However, amongst these remodelers, the INO80 chromatin remodeler appears largely sufficient to generate the well positioned +1 and −1 nucleosomes. S.c INO80 is a multi-subunit complex consisting of 15 subunits that are divided into three different modules. The catalytic module with the Ino80 (ATPase) RecA lobes and insert, Arp5, Ies6, Ies2, Rvb1 and Rvb2, constitutes the core unit of INO80 (C-module). INO80 slides nucleosomes with 40 bp of flanking DNA ~100-fold slower than nucleosomes with 80 bp of flanking DNA, displaying a switch like response to flanking DNA length.

To assess whether the nucleotide state affected the location of the Arp8 module, we determined structures of S.c INO80 on 0/80 and 0/40 nucleosomes in the presence of a non-hydrolysable ATP analog (ADP/BeFx). The overall structure of INO80 bound to 0/80 nucleosomes in the presence of ADP/BeFx is similar to the previously published structure in the apo state. The INO80 C-module is well resolved at a resolution of 2.8 Å. The Arp8 module is resolved as a well-defined density on the flanking DNA (~40 bp). Although at a lower resolution (~11.2 Å), we can dock the previously published atomic model of the S.c Arp8 module bound to the HSA region of the ATPase into this density. For X.l nucleosomes, no difference is observed between the previously published structure in the apo state and the structure determined here in the presence of ADP/BeFx, suggesting that the nucleotide state does not influence the Arp8 module’s conformation on X.l nucleosomes. We further find that for the INO80: X.l 0/80 (ADP/BeFx) sample, a majority of the particles have clear or partial density for the Arp8 module on flanking DNA (classes 2a and 2b) and a small proportion do not show density for the Arp8 module (class 3). In contrast, on 0/80 nucleosomes, where the Arp8 module engages the flanking DNA, this location of the Arp8 module potentially represents a sliding-competent state of INO80.

> MSLAVLLNKEDKDISDFSKTTAGKSAKKNSRERVADVAPTRVLDKKQAYLSQLNSEFNRIKRRDSIEQLYQDWKFINLQEFELISEWNQQSKDWQFDNTNDSQDLHFKKLYRDMSMINKEWAEYQSFKNANLSDIINEKDADEDEEDDEDELEDGEEDMEEDEASTGRHTNGKSMRGNGIQKSRKKDAAAAAAIGKAIKDDQTHADTVVTVNGDENEDGNNGEDEDNDNDNENNNDNDNDNENENDNDSDNDDEEENGEEDEEEEEIEDLDEEDFAAFEEQDDNDDEDFNPDVEKRRKRSSSSSSSTKLSMNSLSLITSKKINKNITINSDRPKIVRELIKMCNKNKHQKIKKRRFTNCIVTDYNPIDSKLNIKITLKQYHVKRLKKLINDAKREREREEALKNNVGLDGNDLDNDEDGSESHKRRKLNNNTANGADDANKRKFNTRHGLPTYGMKMNAKEARAIQRHYDNTYTTIWKDMARKDSTKMSRLVQQIQSIRSTNFRKTSSLCAREAKKWQSKNFKQIKDFQTRARRGIREMSNFWKKNEREERDLKKKIEKEAMEQAKKEEEEKESKRQAKKLNFLLTQTELYSHFIGRKIKTNELEGNNVSSNDSESQKNIDISALAPNKNDFHAIDFDNENDEQLRLRAAENASNALAETRAKAKQFDDHANAHEEEEEEDELNFQNPTSLGEITIEQPKILACTLKEYQLKGLNWLANLYDQGINGILADEMGLGKTVQSISVLAHLAENHNIWGPFLVVTPASTLHNWVNEISKFLPQFKILPYWGNANDRKVLRKFWDRKNLRYNKNAPFHVMVTSYQMVVTDANYLQKMKWQYMILDEAQAIKSSQSSRWKNLLSFHCRNRLLLTGTPIQNSMQELWALLHFIMPSLFDSHDEFNEWFSKDIESHAEANTKLNQQQLRRLHMILKPFMLRRVKKNVQSELGDKIEIDVLCDLTQRQAKLYQVLKSQISTNYDAIENAATNDSTSNSASNSGSDQNLINAVMQFRKVCNHPDLFERADVDSPFSFTTFGKTTSMLTASVANNNSSVISNSNMNLSSMSSNNISNGKFTDLIYSSRNPIKYSLPRLIYEDLILPNYNNDVDIANKLKNVKFNIFNPSTNYELCLFLSKLTGEPSLNEFFRVSTTPLLKRVIERTNGPKNTDSLSFKTITQELLEVTRNAPSEGVMASLLNVEKHAYEREYLNCIQRGYHPNVSAPPVTIEVLGSSHVTNSINNELFDPLISQALSDIPAITQYNMHVKKGIPVEDFPKTGLFPEPLNKNFSSNISMPSMDRFITESAKLRKLDELLVKLKSEGHRVLIYFQMTKMMDLMEEYLTYRQYNHIRLDGSSKLEDRRDLVHDWQTNPEIFVFLLSTRAGGLGINLTAADTVIFYDSDWNPTIDSQAMDRAHRLGQTRQVTVYRLLVRGTIEERMRDRAKQKEQVQQVVMEGKTQEKNIKTIEVGENDSEVTREGSKSISQDGIKEAASALA;> MSSRDASLTPLKAVVIDDPPLRQTPEPFDEQSAYNPQSPIAIDFGSSKLRAGFVNHATPTHIFPNALTKFRDRKLNKNFTFVGNDTLLDQAVRSQSRSPFDGPFVTNWNLTEEILDYTFHHLGVVPDNGIPNPILLTERLATVQSQRTNWYQILFETYNVPGVTFGIDSLFSFYNYNPSGNKTGLVISCGHEDTNVIPVVDGAGILTDAKRINWGGHQAVDYLNDLMALKYPYFPTKMSYLQYETMYKDYCYVSRNYDEDIEKILTLENLDTNDVVVEAPFTEVLQPQKTEEELRIQAEKRKETGKRLQEQARLKRMEKLVQKQEEFEYFSKVRDQLIDEPKKKVLSVLQNAGFDDERDFKKYLHSLEQSLKKAQMVEAEDDSHLDEMNEDKTAQKFDLLDIADEDLNEDQIKEKRKQRFLKASQDARQKAKEEKERVAKEEEEKKLKEQQWRETDLNGWIKDKRLKLNKLIKRRKEKLKLRDEMKDRKSQVSQNRMKNLASLAEDNVKQGAKRNRHQATIDNDPNDTFGANDEDWLIYTDITQNPEAFEEALEYEYKDIVELERLLLEHDPNFTEEDTLEAQYDWRNSILHLFLRGPRPHDSENIHEQHQMHLNVERIRVPEVIFQPTMGGQDQAGICELSETILLKKFGSQPGKLSQTSIDMVNNVLITGGNAKVPGLKERIVKEFTGFLPTGTNITVNMSSDPSLDAWKGMAALARNEEQYRKTVISKKEYEEYGPEYIKEHKLGNTKYFED;> MSGSRGNSSNSSVSNNSNNNNNNDGGDERLLFLRSVGERNEIGFPSRFKSAHYKKPTRRHKSARQLISDENKRINALLTKANKAAESSTAARRLVPKATYFSVEAPPSIRPAKKYCDVTGLKGFYKSPTNNIRYHNAEIYQLIVKPMAPGVDQEYLKLRGANFVLK;>[3x]MVAISEVKENPGVNSSNSGAVTRTAAHTHIKGLGLDESGVAKRVEGGFVGQIEAREACGVIVDLIKAKKMSGRAILLAGGPSTGKTALALAISQELGPKVPFCPLVGSELYSVEVKKTETLMENFRRAIGLRIKETKEVYEGEVTELTPEDAENPLGGYGKTISHVIVGLKSAKGTKTLRLDPTIYESIQREKVSIGDVIYIEANTGAVKRVGRSDAYATEFDLETEEYVPLPKGEVHKKKEIVQDVTLHDLDVANARPQGGQDVISMMGQLLKPKKTEITEKLRQEVNKVVAKYIDQGVAELIPGVLFIDEVNMLDIEIFTYLNKALESNIAPVVVLASNRGMTTVRGTEDVISPHGVPPDLIDRLLIVRTLPYDKDEIRTIIERRATVERLQVESSALDLLATMGTETSLRYALQLLAPCGILAQTSNRKEIVVNDVNEAKLLFLDAKRSTKILETSANYL;>[3x]MSIQTSDPNETSDLKSLSLIAAHSHITGLGLDENLQPRPTSEGMVGQLQARRAAGVILKMVQNGTIAGRAVLVAGPPSTGKTALAMGVSQSLGKDVPFTAIAGSEIFSLELSKTEALTQAFRKSIGIKIKEETELIEGEVVEIQIDRSITGGHKQGKLTIKTTDMETIYELGNKMIDGLTKEKVLAGDVISIDKASGKITKLGRSFARSRDYDAMGADTRFVQCPEGELQKRKTVVHTVSLHEIDVINSRTQGFLALFTGDTGEIRSEVRDQINTKVAEWKEEGKAEIVPGVLFIDEVHMLDIECFSFINRALEDEFAPIVMMATNRGVSKTRGTNYKSPHGLPLDLLDRSIIITTKSYNEQEIKTILSIRAQEEEVELSSDALDLLTKTGVETSLRYSSNLISVAQQIAMKRKNNTVEVEDVKRAYLLFLDSARSVKYVQENESQYIDDQGNVQISIAK;> MDSEASDIEAELSDSVSAGGEEYIDDDDYTEDIDDQIVTAKSSRRTARRSVPKGVRTSKRIRDKELSVEVDEDYDEEEDVLSPSKKRHLHTRSMDKRQVAATASEKSDIGDSKGNDGEIEDGILEEEESLEKELNRGGGKEVEKSEESYYAQNDVGQKGEEEQDGESGGYEDNEPSISKESDELVSVVNGNGNEEDDEVEATKENTTDSTRSTTTRSKMLLDLLEDGGSKKKLTDEEIQLRRAENARKRKNLSEKRLEEEKQDTINKLLKKRAGKSRSHLPNDDEKNDGSSSFVKPRRPYNSEGMTRILRRYEEDLFCTF The Phox homology (PX) domain was first identified in the NADPH phagocyte oxidase complex subunits p40phox and p47phox, and has since been found in proteins in every eukaryotic species from yeast to human. Despite relatively low overall sequence homology, PX domains all possess the same core fold, consisting of three antiparallel β-strands (β1-β3), followed by three α-helices (α1–α3). An extended sequence traverses the protein between helices α1 and α2, termed the PPK loop as it generally contains a conserved ΨPxxPxK motif (Ψ = large aliphatic amino acids V, I, L, and M). Side chains of residues from the β3 strand, α1 helix and PPK loop together form a binding pocket for the headgroup of the canonical lipid PtdIns3P.

We have also obtained two crystal structures of SGK3 and SNX23 (for which previous structures exist), as well as a crystal structure of SNX15, the crystal structure of SNX32 (in complex with a peptide from the bacterial IncE peptide) and the NMR structure of SNX25. PX domains are found in a wide variety of proteins with diverse functions, including cell signalling (e.g., PLD1 and 2, PIKC2α, β, and γ), vesicle trafficking (e.g., SNXs 1, 2, 3, 5, and 6), protein scaffolding (e.g., SH3PXD2A and B), and cytoskeletal transport (SNX23/KIF16B).

>GSDPIKISIPRYVLCGQGKDAHFEFEVKITVLDETWTVFRRYSRFREMHKTLKLKYAELAALEFPPKKLFGNKDERVIAERRSHLEKYLRDFFSVMLQSATSPLHINKVGLTLSKHTICEFSPFFKKGVFDYS[3x]>MAASQEIFLQVLNLADGDVKVTVLGSRNNSLLVESVSSFQNTTHYSKLHLEAKSQDLHFHLKYNSLSVHNDHSVEEKNCYQLLIHQDGESISSMLVKDTGIKPANGMAAIRFINTLHKDLNISLDTDAPLSVGKDYGVSAYRTVLRGKYPAVHCETEDKVFSLDLGQLDFGTTYLFVITNITSQGLQAWKAEDI[3x]

Mammals obtain nitrogen via the uptake of di- and tri-peptides in the gastrointestinal tract through the action of PepT1 and PepT2, which are members of the POT family of proton-coupled oligopeptide transporters. However, a key structural difference exists between bacterial and mammalian homologs with only the latter containing a large extracellular domain, the function of which is currently unknown. Here, we present the crystal structure of the extracellular domain from both PepT1 and PepT2 that reveal two immunoglobulin-like folds connected in tandem, providing structural insight into mammalian peptide transport. Functional and biophysical studies demonstrate that these domains interact with the intestinal protease trypsin, suggesting a role in clustering proteolytic activity to the site of peptide transport in eukaryotic cells.

Following extensive screening, crystals from Rattus norvegicus PepT2, residues 410–601, were also obtained. The phases were calculated from seleno-L-methionine incorporated protein using the SAD method in space group P3221. A higher-resolution structure in space group P41212 was obtained using the P3221 crystals as seeds with a single monomer in the asymmetric unit. The crystal structures revealed that in the PepT1ECD there exist two conserved salt bridge interactions stabilizing the interface between lobe 1 and lobe 2, mediated by Asp574-Lys398 and Asp476-Arg490, whereas in PepT2ECD only one equivalent salt bridge interaction is present, between Asp505 and Arg538. Guinier analysis of the scattering data in PRIMUS (Petoukhov et al., 2007) shows that PepT2ECD has a larger radius of gyration (Rg) compared with PepT1ECD, 23.1 versus 18.4 Å, which suggests an increase in particle size. Consistent with this analysis, 3D envelopes of the ECD generated using DAMMIF show that PepT1ECD forms a compact shape ∼48 Å in length whereas PepT2ECD is more elongated, approximately 61 Å in length. The larger envelope of PepT2ECD indicates that the two immunoglobulin-like domains are structurally more dynamic than the PepT1ECD, which is consistent with the loss of the second salt bridge and also the location of Asp505 on the unstructured loop connecting lobes 1 and 2. From this panel of potential ligands we observed binding only for the intestinal protease trypsin with both mouse PepT1ECD (KD 80 ± 0.8 μM) and rat PepT2ECD (KD 165 ± 0.5 μM). We identified two highly conserved charged residues, Asp550 and Glu573 in PepT1ECD and Asp576 and Glu599 in PepT2ECD, located on one face of the ECD structure.> YFQGHMMIHAPRRWV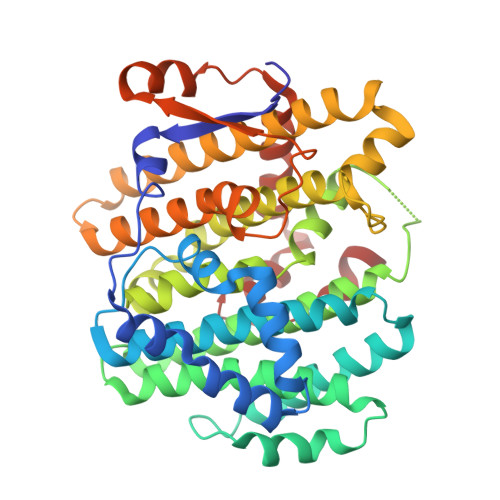ERHKQVQVLPQNAVEKLISMNELIELVIECGLCDKTSIKKMYDKINTYQFMWCIVDTIPASQYAEEIFKSSLHFLCALFLVDDAVESYSANEMQDLSRSYDILEKEVCKTFPNFPSINEMKESLMHLRNPFDRSSITFCMQYVNKITAILLEEGNTPHHVVYNLRRRTSNAISIAFQAVLIKSKCGSIITSHEMLWRRVFDGLVILFYQFGELISGATETAQQHITVVTELRMLGCLYCIVINDLYSYQRDKLASSDNMIKTWLLEKTVSSLSEATARCSQILDAIMKYMYQRVEQCMQSNPGCPQLESLLETTIYTTVGWIRSHTTVVPRYSESQLKVALVEVEERELPKWLAEKDEYGWNVVEKFVETLNDEKHKGILDALQGIADGRDQLLKTQ>[5x]MGSDKIHHHHHHMFYEIRTYRLK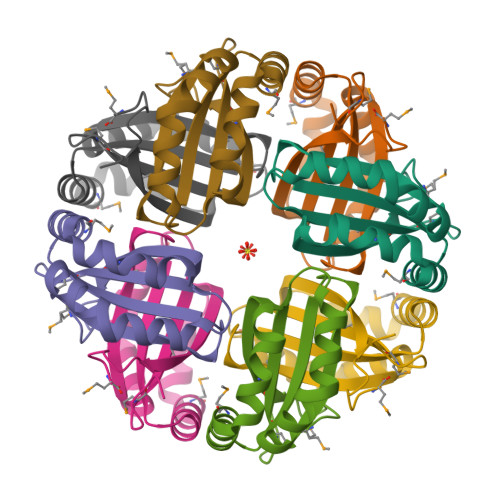NGAIPAYLKVVEDEGIEIQKSHLGELVGYFFSEIGPINEIVHIWAFSSLDDRAERRARLMADPRWLSFLPKIRDLIEVAENKIMKPARFSPLM>[2x]MASHHHHHHHHHHENLYFQGSKRHIPVVTDIYSVEDHRLEDTTHLQYAPNAIKTEGKGSGSGPAVCKKVTEHERCTTSIMDKLTAFFGVMPRGTTPRAPVRFPTSLLKIRRGLETGWAYTHQGGISSVDHVTCGKDLLVCDTMGRTRVVCQSNNKMTDESEYGVKTDSGCPEGARCYVFNPEAVNISGTKGAMVHLQKTGGEFTCVTASGTPAFFDLKNLKGWAGLPIFEASSGRVVGRVKVGKNEDSKPTKLMSGIQTVSKSATDLTEMVKKITTMNRGEFRQITLATGAGKTTELPRSVIEEIGRHKRVLVLIPLRAAAESVYQYMRQKHPSIAFNLRIGEMKEGDMATGITYASYGYFCQMSQPKLRAAMVEYSFIFLDEYHCATPEQLAIMGKIHRFSENLRVVAMTATPAGTVTTTGQKHPIEEFIAPEVMKGEDLGSEYLDIAGLKIPVEEMKNNMLVFVPTRNMAVEAAKKLKAKGYNSGYYYSGEDPSNLRVVTSQSPYVVVATNAIESGVTLPDLDVVVDTGLKCEKRIRLSPKMPFIVTGLKRMAVTIGEQAQRRGRVGRVKPGRYYRSQETPVGSKDYHYDLLQAQRYGIEDGINITKSFREMNYDWSLYEEDSLMITQLEILNNLLISEELPMAVKNIMARTDHPEPIQLAYNSYETQVPVLFPKIRNGEVTDTYDNYTFLNARKLGDDVPPYVYATEDEDLAVELLGLDWPDPGNQGTVEAGRALKQVVGLSTAENALL

The cleavages downstream of NS3, NS4A, NS4B and NS5A are catalyzed by the serine protease domain of NS3 which requires NS4A as cofactor for full proteolytic activity and is termed NS3-4A protease. In addition to its protease function, NS3 of HCV and pestiviruses comprises helicase and NTPase activity. Co-immunoprecipitation experiments have shown that NS4A forms a stable complex with NS3 (NS3/4A complex). In view of the critical role of the NS3/4A protein complex in the switch between RNA replication and virion assembly, the determination of the structure of a single-chain CSFV NS3 serine protease-NS4A complex provided the basis for structure-guided functional analyses.

We report here the crystal structure of a single chain construct encompassing full-length pestivirus NS3 in complex with NS4A residues 21–57. To express soluble CSFV NS4A37NS3 for crystallization, we used recombinant constructs encoding full-length NS3 (residues 1 to 683) followed by the 8 N-terminal residues of NS4A; the NS3 sequence is preceeded by residues 21 to 57 of the protease cofactor NS4A. Like in the crystals of the isolated NS3 helicase domain, the two molecules of NS4A37NS3 present in the asymmetric unit (AU) are related by a local 2-fold axis around the helicase domains in which D1 and D3 make a head-to-tail crystallographic dimer interaction. Within a pair, one molecule adopts an elongated conformation (Zmax = 105 Å) similar to what has been observed for different flavivirus NS3 proteins and the other, a more compact conformation (Zmax = 69 Å), similar to HCV NS3 depending on the different orientations of the protease domain relative to the helicase domain. The overall shape of the pestiviral NS4A37NS3 is very similar to its counterparts from the Flavivirus and Hepacivirus genera with two separate globular domains, representing the protease and helicase, linked by a short flexible interdomain region that explains the different relative orientations of the two domains in our structures. The CSFV NS3pro domain, which comprises 192 residues, shares only 3% of sequence identity among the NS3 proteases within the Flaviviridae family. It has the canonical trypsin-like fold containing two β-barrels, with the conserved Asp-His-Ser catalytic triad located in a cleft between them. Like in hepaciviral- and flaviviral proteases, the pestiviral NS3 protease domain seems also to be stabilized by the insertion of a β-sheet from NS4A (residues 21 to 40). Most interestingly, the C-terminal region of the pestivirus NS4A, namely residues 41 to 49, hereafter referred to as "kink region", is interacting with a hydrophobic patch on the surface of NS3pro. Interestingly, residue 132, a methionine in the closely related CSFV (valine in BVDV) and most other pestivirus strains is located on the NS3 protease surface and makes hydrophobic contacts mainly with L45 of the NS4A-kink region.> C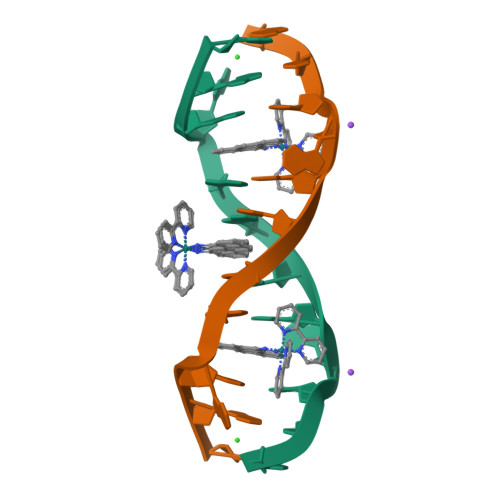GGAAATTACCG> HSLGKDDLRPSSPLLSVFGVLILTLLGFLVAATFAWNLLVLATILRVRTFHRVPHNLVASMAVSNVLVAALVMPLSLVHELSGRRWQLGRRLCQLWIACDVLCCTASIWNVTAIALDRYWSITRHMEYTLRTRKCV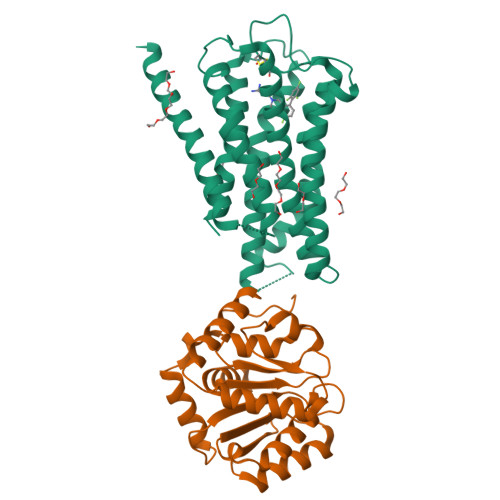SNVMIALTWALSAVISLAPLLFGWGETYSEGSEECQVSREPSYAVFSTVGAFYLPLCVVLFVYWKIYKAAKFRVGSRKTNSVSPISEAVEVKDSAKQPQMVFTVRHATVTFQPEGDTWREQKEQRAALMVGILIGVFVLCWAPFFLTELISPLCSCDIPAIWKSIFLWLGYSNSFFNPLIYTAFNKNYNSAFKNFFSRQH;> GSHNGIDCSFWNESYLTGSRDERKKSLLSKFGMDEGVTFMFIGRFDRGQKGVDVLLKAIEILSSKKEFQEMRFIIIGKGDPELEGWARSLEEKHGNVKVITEMLSREFVRELYGSVDFVIIPSYFEPFGLVALEAMCLGAIPIASAVGGLRDIITNETGILVKAGDPGELANAILKALELSRSDLSKFRENCKKRAMSFS>ATPADWRSQSIYFLLTDRFARTDGSTTATCNTADQKYCGGTWQGIIDKLDYIQGMGFTAIWITPVTAQLPQDCAYGDAYTGYWQTDIYSLNENYGTADDLKALSSALHERGMYLMVDVVANHMGYDGAGSSVDYSVFKPFSSQDYFHPFCFIQNYEDQTQVEDCWLGDNTVSLPDLDTTKDVVKNEWYDWVGSLVSNYSIDGLRIDTVKHVQKDFWPGYNKAAGVYCIGEVLDGDPAYTCPYQNVMDGVLNYPIYYPLLNAFKSTSGSMDDLYNMINTVKSDCPDSTLLGTFVENHDNPRFASYTNDIALAKNVAAFIILNDGLPIIYA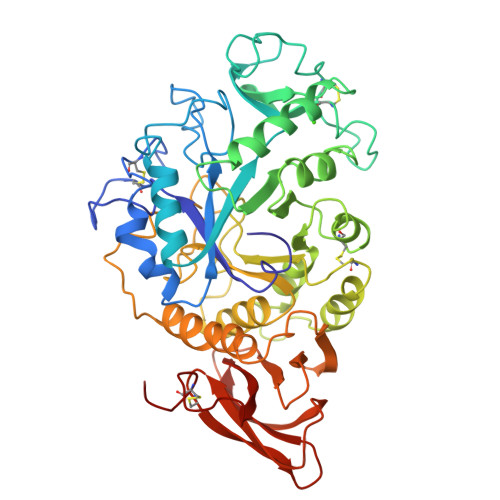GQEQHYAGGNDPANREATWLSGYPTDSELYKLIASANAIRNYAISKDTGFVTYKNPYIKDDTTIAMRKGTDGSQIVTILSNKGASGDSYTLSLSGASYTAGQQLTEVIGCTTVTVGSDGNVPVPMAGGLPRVLYPTEKLAGSKICSDSS[3x]> XKKRYSRLQLLLFW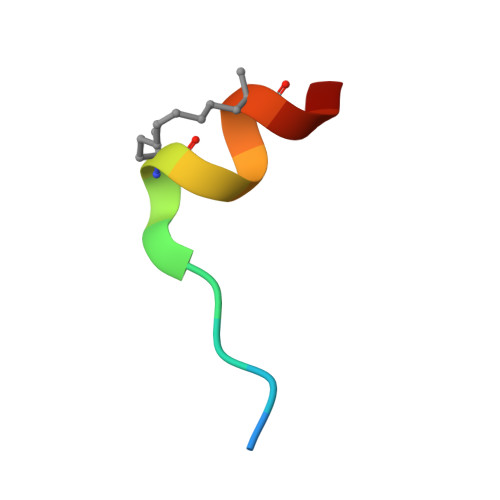X> VNQSETPVKHIGKIFFTLGGSNYVCSGNSVTAANKSTVSTAGHCLNEGPGAYATNFIFVPAYLNGAAP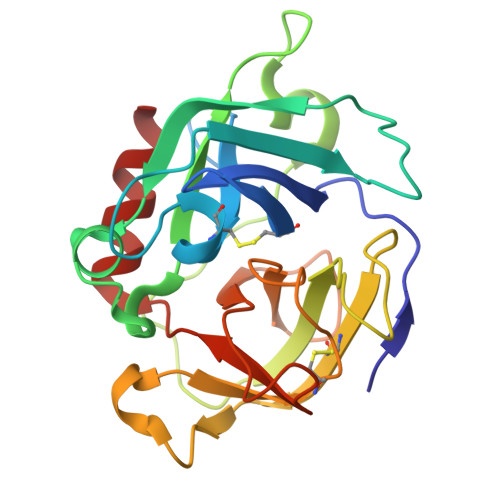YGKWTAKALYAPTQWASNGNMQYDTAFAVMNTLNGQKLADVVGSSGVQFNAARGLSYKSFGYPAASPFNGESLKSCSGTATNDPYNPQFATQGIPCNMTGGSSGGPWFIGNSSSGYQNSVNSYGYGSNSSTMYGPYWGTVIQSTYNTAAAS1-(trifluoromethyl)cyclobutyl {(2R,4S,6S,12Z,13aS,14aR,16aS)-2-[(7-methoxy-3-methylquinoxalin-2-yl)oxy]-14a-[(1-methylcyclopropane-1-sulfonyl)carbamoyl]-5,16-dioxo-1,2,3,5,6,7,8,9,10,11,13a,14,14a,15,16,16a-hexadecahydrocyclopropa[e]pyrrolo[1,2-a][1,4]diazacyclopentadecin-6-yl}carbamate 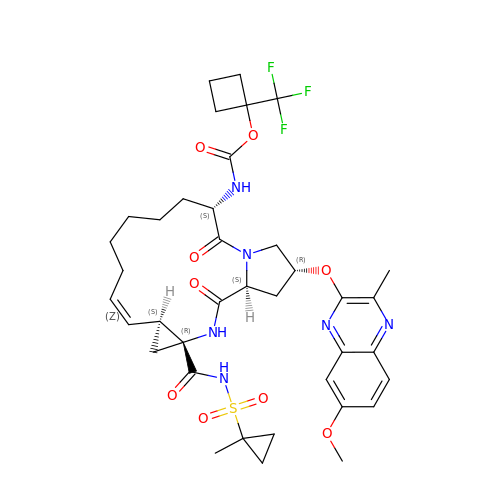| C38 H47 F3 N6 O9 S | RXAPCCHAKDPLNB-ZEJZJNHJSA-N> GPALVDADDVMTKEEQIFLLHRAQAQCEKRLKEVLQRPAGRPCLPEWDHILCWPLGAPGEVVAVPCPDYIYDFNHKGHAYRRCDRNGSWELVPGHNRTWANYSECVKFLTNETREREVFDRLGMICTVGYSVSLASLTVAVLILAYFRRLHCTRNYIHMHLFLSFMLRAVSIFVMDAVLYSGATLDEAERLTEEELRAIAQAPPPPATAAAGYAGCRVAVTFFLYFLATNYYWIAVEGLYLHSLIFKAFFSEKKYLWGFTVFGWGLPAIFVAVWVSVRATLANTGCWDLSSGNNKWIIQVPILASIVLNFILFINIVRVLATKGIDCSFWNESYLTGSRDERKKSLLSKFGMDEGVTFMFIGRFDRGQKGVDVLLKAIEILSSKKEFQEMRFIIIGKGDPELE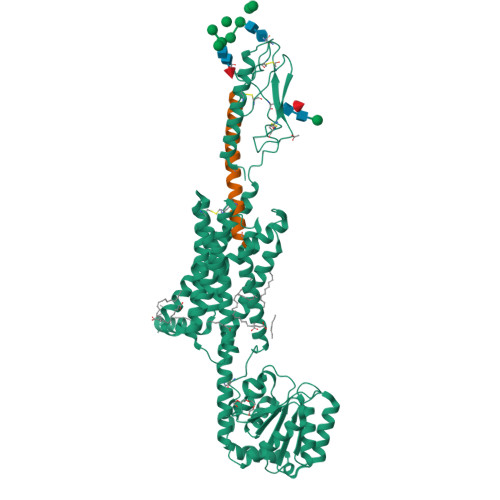GWARSLEEKHGNVKVITEMLSREFVRELYGSVDFVIIPSYFEPFGLVALEAMCLGAIPIASAVGGLRDIITNETGILVKAGDPGELANAILKALELSRSDLSKFRENCKKRAMSFSDTRQQYRKLAKSTLVLMPLFGVHYIVFMLTPYTEVSGTLWQVRMHYEMLFNSFQGFFVAIAYCFCNGEVQAEIKKSWSRWTLA;> XVAEIQLMHQRAKWLNSLERVEWLRKKLQDVHNYX>[4x]GGCUGGGUUUUUC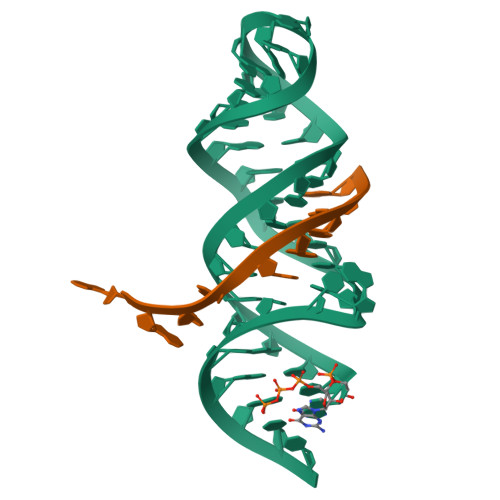CUUCGAAAGAAGGUUUUUAUCCCAGUC;>AAAAAAAAA[4x]> 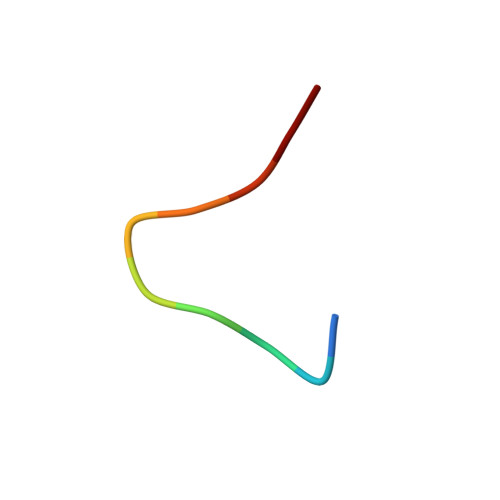MYWYPYASGS>MSVPKKRNHGKLPPSTKDVDDPSLKYTKAAPKCEQVAEHWLLQPLPEPESRYSFWVTIVTLLAFAARFYKIWYPKEVVFDEVHFGKFASYYLERSYFFDVHPPFAKMMIAFIGWLCGYDGSFKFDEIGYSYETHPAPYIAYRSFNAILGTLTVPIMFNTLKELNFRAITCAFASLLVAIDTAHVTETRLILLDAILIISIAATMYCYVRFYKCQLRQPFTWSWYIWLHATGLSLSFVISTKYVGVMTYSAIGFAAVVNLWQLLDIKAGLSLRQFMRHFSKRLNGLVLIPFVIYLFWFWVHFTVLNTSGPGDAFMSAEFQETLKDSPLSVDSKTVNYFDIITIKHQDTDAFLHSHLARYPQRYEDGRISSAGQQVTGYTHPDFNNQWEVLPPHGSDVGKGQAVLLNQHIRLRHVATDTYLLAHDVASPFYPTNEEITTVTLEEGDGELYPETLFAFQPLKKSDEGHVLKSKTVSFRLFHVDTSVALWTHNDELLPDWGFQQQEINGNKKVIDPSNNWVVDEIVNLDEVRKVYIPKVVKPLPFLKKWIETQKSMFEHNNKLSSEHPFASEPYSWPGSLSGVSFWTNGDEKKQIYFIGNIIGWWFQVISLAVFVGIIVADLITRHRGYYAL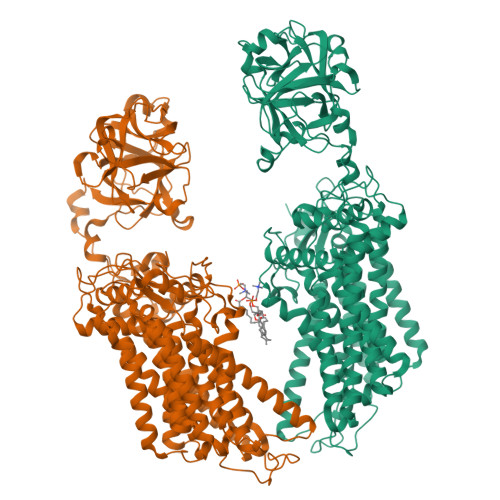NKMTREKLYGPLMFFFVSWCCHYFPFFLMARQKFLHHYLPAHLIACLFSGALWEVIFSDCKSLDLEKDEDISGASYERNPKVYVKPYTVFLVCVSCAVAWFFVYFSPLVYGDVSLSPSEVVSREWFDIELNFSK[2x]>GAMEGGAGAAASRALQQCGQLQKLIDISIGSLRGLRTKCAVSNDLTQQEIRTLEAKLVRYICKQRQCKLSVAPGERTPELNSYPRFSDWLYTFNVRPEVVQEIPRDLTLDALLEMNEAKVKETLRRCGASGDECGRLQYALTCLRKVT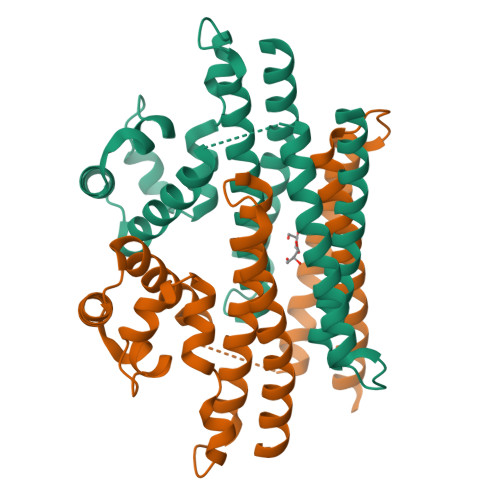GGSGSGSGSSSAADPAIPEEVWNIKQMIKLTQEHIEALLDKFGGEHNPPSIYLEAYEEYTSKLDALQQREQQLLESLGNGTDFS[2x]> SLTDSVYERLLSERIIFLGSEVNDEIANRLCAQILLLAAEDASKDISLYINSPGGSISAGMAIYDTMVLAPCDIATYAMGMAASMGEFLLAAGTKGKRYALPHARILMHQPLGGVTGSAADIAIQAEQFAVIKKEMFRLNAEFTGQPIERIEADS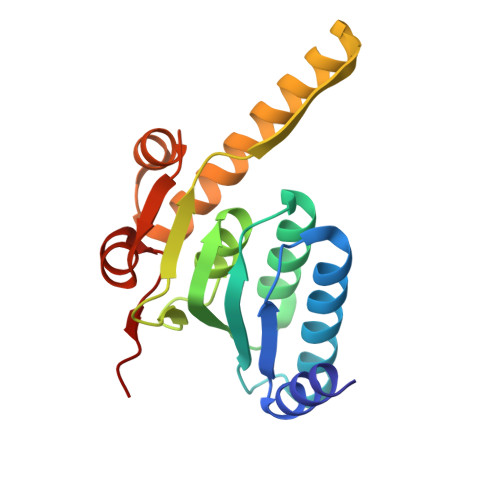DRDRWFTAAEALEYGFVDHIITR>MVDPVGFAEAWKAQFPDSEPPRMELRSVGDIEQELERAKASIRRLEQEVNQERFRMIYLQTLLAKEKKS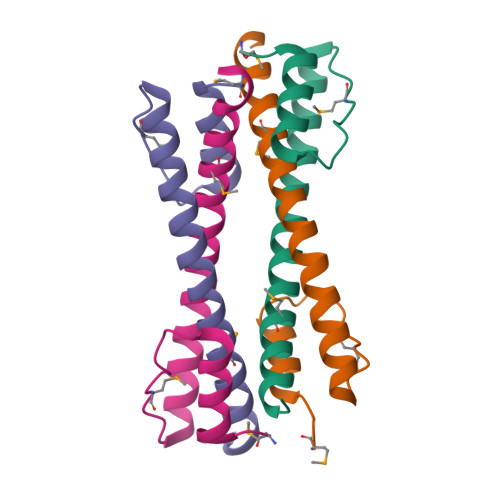YDR[8x]>MRVGIPTETKNNEFRVAITPAGVAELTRRGHEVLIQAGAGEGSAITDADFKAAGAQLVGTADQVWADADLLLKVKEPIAAEYGRLRHGQILFTFLHLAASRACTDALLDSGTTSIAYETVQTADGALPLLAPMSEVAGRLAAQVGAYHLMRTQGGRGVLMGGVPGVEPADVVVIGAGTAGYNAARIANGMGATVTVLDINIDKLRQLDAEFCGRIHTRYSSAYELEGAVKRADLVIGAVLVPGAKAPKLVSNSLVAHMKPGAVLVDIAIDQGGCFEGSRPTTYDHPTFAVHDTLFYCVANMPASVPKTSTYALTNATMPYVLELADHGWRAACRSNPALAKGLSTHEGALLSERVATDLGVPFTEP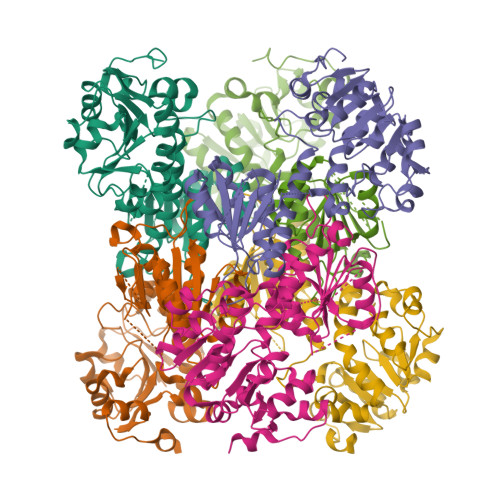ASVLAHHHHHH[2x]Human bestrophin1 (hBest1) is a Ca2+-activated Cl− channel essential for Cl− transport in retinal pigment epithelium (RPE). Although the structure of hBest1 is still unsolved, two Best1 homolog structures, one from bacteria Klebsiella pneumoniae (KpBest) and the other from chicken (cBest1), have been previously reported. Overall, the channel is a pentameric assembly with a single ion-conducting pathway, which varies in diameter along its length and is constrained at two narrow points: a “neck” contributed by three residues (I62/I66/F70 in KpBest and I76/F80/F84 in hBest1/cBest1) on a transmembrane helix, and an “aperture” formed by a single residue (I180 in KpBest1, I205 in hBest1, and V205 in cBest1) on a cytosolic helix. Here, by electrophysiological and structural analyses, we show that the neck and aperture in hBest1 are both indispensable Ca2+-dependent gates, and their dysregulated opening by rationally designed or patient-derived mutations causes Ca2+-independent leak and elevates Ca2+-dependent channel activity.

In KpBest and hBest1, alanine substitution at the aperture (KpBest I180A and hBest1 I205A) significantly enhanced channel activity, suggesting an activation gate role for the aperture. To characterize how alanine substitution affects the size of the aperture, we solved the crystal structure of the KpBest I180A mutant (equivalent to hBest1 I205A) at 2.9 Å. Compared to WT KpBest, the I180A mutant displays a much bigger opening at the aperture (radius 0.9 vs. 3.2 Å) without altering the overall structure of the channel (RMSD = 0.4 Å). Notably, the structure of this region is well preserved among species, providing a molecular basis for dehydrated Cl− and CH3SO3− (radius 1.8 and 2.6 Å, respectively) to pass through the aperture of hBest1 I205A in the absence of Ca2+. Consistent with this idea, KpBest I180A (equivalent to hBest1 I205A) displayed dramatically increased open probability but unchanged unitary current in lipid bilayer. While mutants with conformational changes at the aperture (e.g., KpBest I180A, I180T) or neck (e.g., cBest1 3A) do not have structural alteration at the other restriction, a mutation near the aperture (D203A and D179A in hBest1 and KpBest, respectively) impacts both gates, suggesting both independent and cooperative regulations of the two channel gates. The hBest1 4A mutant is designed to be deficient in gating at both the neck and aperture, because the cBest1 3A and KpBest I180A mutant exhibit an unconstrained neck and aperture for Cl−, respectively.

>[5x]NAMIIRPEQHWFLRLFDWHGSVLSKIIFRLLLNVLMSIIAIISYQWYEQLGIHLTVAPFSLLGIAIAIFLGFRNSASYSRFVEARNLWGTVLIAERTLVRQLRNILPAEHDAHRRIVSYLVAFSWSLKHQLRKTDPTADLRRLLPEERVTEILASSMPTNRILLLAGNEIGQLREAGKLSDATYGLMDNKLDELAHVLGGCERLATTPVPFAYTLILQRTVYLFCTLLPFALVGDLHYMTPFVSVFISYTFLSWDSLAEELEDPFGTAANDLPLNAMCNTIERNLLDMTGQHPLPE>[10x]PVDVSVSIFINKIYGVNTLEQTYKVDGYIVAQWTGKPRKTPGDKPLIVENTQIERWINNGLWVPALEFINVVGSPDTGNKRLMLFPDGRVIYNARFLGSFSNDM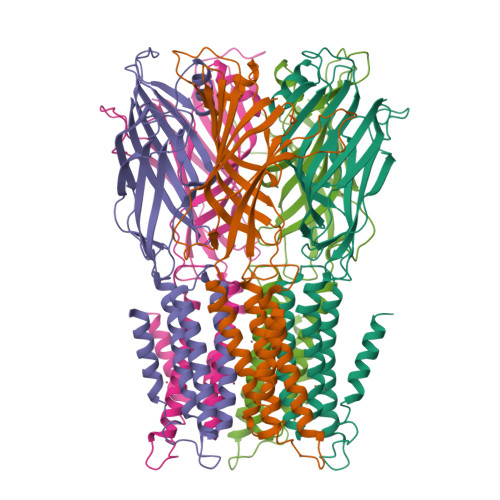DFRLFPFDRQQFVLELEPFSYNNQQLRFSDIQVYTENIDNEEIDEWWIRGKASTHISDIRYDHLSSVQPNQNEFSRITVRIDAVRNPSYYLWSFILPLGLIIAASWSVFWLESFSERLQTSFTLMLTVVAYAFYTSNILPRLPYTTVIDQMIIAGYGSIFAAILLIIFAHHRQANGVEDDLLIQRCRLAFPLGFLAIGCVLVI>MAVSTVTGAAGIGLATLAADGSVLDTWFPAPELTESGTSATSRLAVSDVPVELAALIGRDDDRRTETIAVRTVIGSLDDVAADPYDAYLRLHLLSHRLVAPHGLNAGGLFGVLTNVVWTNHGPCAIDGFEAVRARLRRRGPVTVYGVDKFPRMVDYVVPTGVRIADADRVRLGAHLAPGTTVMHEGFVNYNAGTLGASMVEGRISAGVVVGDGSDVGGGASIMGTLSGGGTHVISIGKRCLLGANSGLGISLGDDCVVEAGLYVTAGTRVTMPDSNSVKARELSGSSNLLFRRNSVSGAVEVLARDGQGIALNEDLHANGVPRGLEHHHHHH[5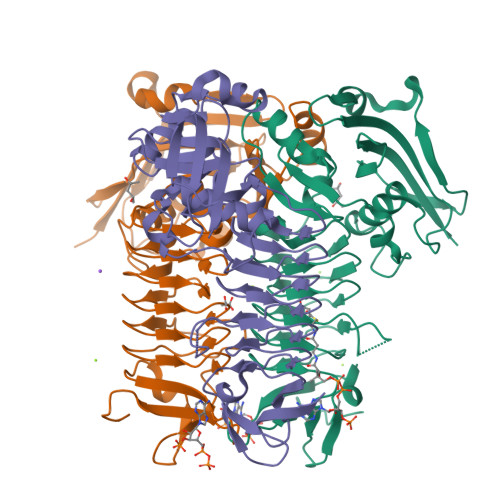x]4-[(1-oxidanyl-3~{H}-2,1-benzoxaborol-5-yl)oxy]benzaldehyde 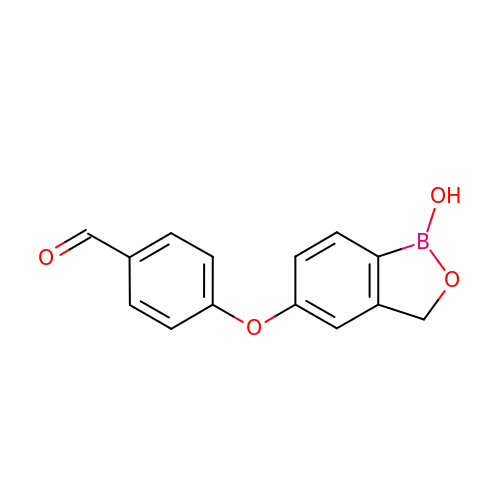| C14 H11 B O4 | HSAPOLFXQLNVEC-UHFFFAOYSA-N> GDPIADMIDQTVNNQVNRSLTALQVLPTAANTEASSHRLGTGVVPALQAAETGASSNASDKNLIETRCVLNHHSTQETAIGNFFSRAGLVSIITMPTTGTQNTDGYVNWDIDLMGYAQLRRKCELFTYMRFDAEFTFVVAKPNGELVPQLLQYMYVPPGAPKPTSRDSFAWQTATNPSVFVKMTDPPAQVSVPFMSPASAYQWFYDGYPTFGEHLQANDLDYGQCPNNMMGTFSIRTVGIEKSPHSITLRVYMRIKHVRAWIPRPLRNQPYLFKTNPNYKGNDIKCTSTSRDKITTL;> SPSAEACGYSDRVAQLTIGNSTITTQEAANIVIAYGEWPEYCPDTDATAVDKPTRPDVSVNRFFTLDTKSWAKDSKGWYWKFPDVLTEVGVFGQNAQFHYLYRSGFCVHVQCNASKFHQGALLVAVLPEYVLGTIAGGTGNENSHPPYATTQPGQVGAVLTHPYVLDAGIPLSQLTVCPHQWINLRTNNCATIIVPYMNTVPFDSALNHCNFGLLVIPVVPLDFNTGATSEIPITVTIAPMCAEFAGLRQAVKQ;> GIPTELKPGTNQFLTTDDGVSAPILPGFHPTPPIHIPGEVHNLLEICRVETILEVNNLKTNETTPMQRLCFPVSVQSKTGELCAAFRADPGRDGPWQSTILGQLCRYYTQWSGSLEVTFMFAGSFMATGKMLIAYTPPGGNVPADRITAMLGTHVIWDFGLQSSVTLVVPWISNTHYRAHARAGYFDYYTTGIITIWYQTNYVVPIGAPTTAYIVALAAAQDNFTMKLCKDTEDIEQTANIQ;> MGSQVSTQRSGSHENSNSASEGSTINYTTINYYKDAYAASAGRQDMSQDPKKFTDPVMDVIHEMAPPLK

Enterovirus 71 (EV71) and coxsackievirus A16 (CVA16) are subgroup A human enteroviruses (HEVA), small, nonenveloped single-stranded RNA (ssRNA) viruses whose protective capsid mediates cell entry and humoral immune responses. The external portion of the icosahedral capsid comprises 60 copies of viral proteins VP1, -2, and -3 arranged with pseudo T=3 symmetry, while their N-terminal extensions and 60 copies of VP4 line the interior, surrounding the RNA genome. There is a “canyon” (a depression encircling the 5-fold axes) on the surface of enteroviruses that often harbors the receptor binding site, and there is a fatty acid binding site below the canyon base, within the hydrophobic β-barrel core of VP1. Here, we remedy this with high resolution X-ray structures of both mature and natural empty CVA16 particles and also of empty recombinant viruslike particles of CVA16 produced in insect cells, a potential vaccine antigen.

CVA16 (strain Ningbo.CHN/028-2/2009) was grown in Vero cells and formaldehyde inactivated prior to purification. The sedimentation coefficients and λ260/λ280 absorbance ratios were ∼160S and 1.67 for the mature virus, and ∼80S and 0.64 for the empty particle, indicating that the latter does not contain RNA, and SDS-PAGE showed that VP0 is not cleaved into VP4 and VP2 in the empty particle. Diffraction data for inactivated CVA16 empty and full virus particles to 2.7- and 2.65-Å resolution, respectively, were collected at room temperature in situ. The crystals of both mature and empty particles belong to the same space group, P41212, with similar unit cell dimensions of a = b = 491 Å and c = 709 Å. The mature CVA16 virus particle contains VP1 to -4 and is well ordered apart from residues 1 and 9 to 17 of VP1, 1 to 9 of VP2, and 1 to 11 of VP4. Given ∼80% identity (with no insertions or deletions) in the capsid protein sequences of CVA16 and EV71, it is unsurprising that their overall structures are very similar; 823 Cα out of 832 match with a root mean square deviation (RMSD) of 0.5 Å. The most significant differences are on the outer surface, including the BC loop and C-terminal residues 280 to 297 of VP1 and, in VP3, residues 58 to 66 leading to the B strand and the C-terminal residues 233 to 239. Thus, residues 59 to 62 and 65 to 69 of VP3 form 2 short helices linked by a tight turn in CVA16, compared to a loop and a longer helix (62 to 69) in EV71. The inner surface of the CVA16 particle is similar to that of EV71 and distinct from those of other known enteroviruses: VP1 starts adjacent to the icosahedral 2-fold axis underneath the αA helix of VP2 and folds across the protomer, while residues 12 to 31 of VP4 form a loose spiral beneath VP1. VP1 contains a bound pocket factor, modeled as sphingosine (similar to EV71).5-ethyl-2-(phenylcarbonyl)imidazo[1,2-a]pyrimidin-7(1H)-one | C15 H13 N3 O2 | 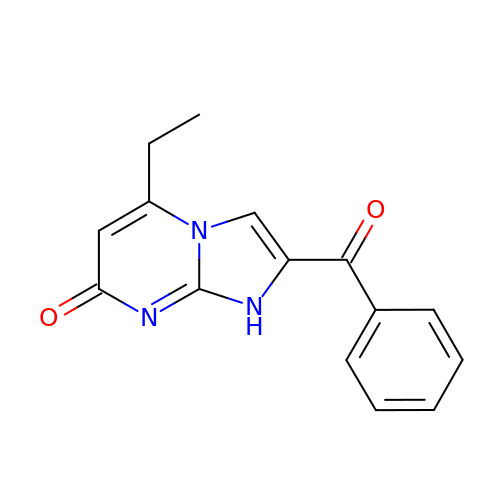VHONGMGMJIQAAN-UHFFFAOYSA-N>MTDLNIPHTHAHLVDAFQALGIRAGQALMLHASVKAVGAVMGGPNVILQALMDALTPDGTLMMYAGWQDIPDFIDSLPDALKAVYLEQHPPFDPATARAVRENSVLAEFLRTWPCVHRSANPEASMVAVGRQAALLTANHALDYGYGVESPLAKLVAIEGYVLMLGAPLDTITLLHHAEYLAKMRHKNVVRYPCPILRDGRKVWVTVEDYDTGDPHDDYSFEQIARDYVAQGGG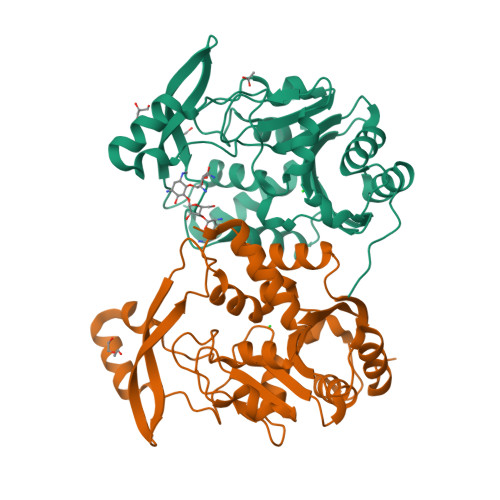TRGKVGDADAYLFAAQDLTRFAVQWLESRFGDSAS[2x]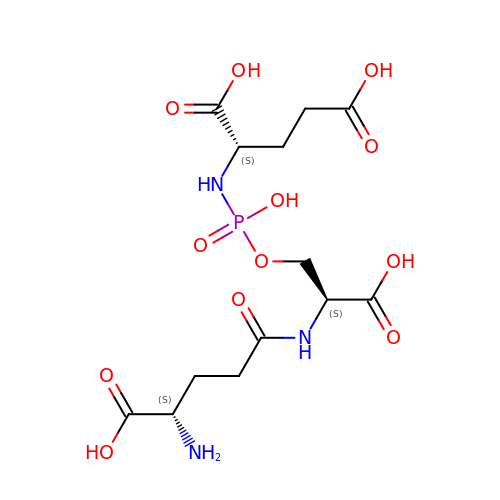L-gamma-glutamyl-O-[(S)-{[(1S)-1,3-dicarboxypropyl]amino}(hydroxy)phosphoryl]-L-serine | C13 H22 N3 O12 P | KSAFNYJPIDGLBS-FXQIFTODSA-N> GSHMDYLVTEEEINLTRGPSGLGFNIVGGTDQQYVSNDSGIYVSRIKENGAAALDGRLQEGDKILSVNGQDLKNLLHQDAVDLFRNAGYAVSLRVQHRLQVQGSAYGSVKAYTNFDAERDALNIETAIKTKGVDEVTIVNILTNRSNEQRQDIAFAYQRRTKKELASALKSALSGHLETVILGLLKTPAQYDASELKASMKGLGTDEDSLIEIICSRTNQELQEINRVYKEMYKTDLEKDIISDTSGDFRKLMVALAKGRRAEDGSVIDYELIDQDARDLYDAGVKRKGTDVPKWISIMTERSVPHLQKVFDRYKSYSPYDMLESIRKEVKGDLENAFLNLVQCI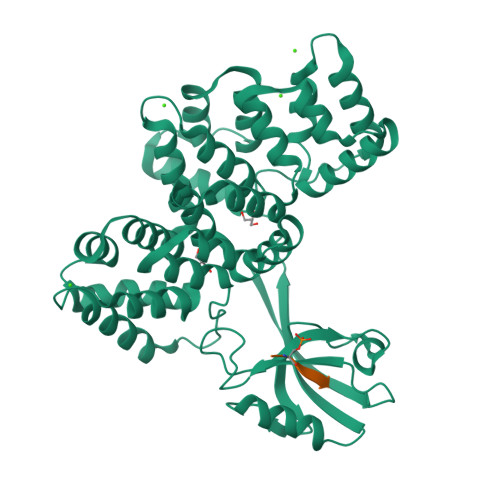QNKPLYFADRLYDSMKGKGTRDKVLIRIMVSRSEVDMLKIRSEFKRKYGKSLYYYIQQDTKGDYQKALLYLCGGDD;> TDDSRRVRKLPSTTL> MA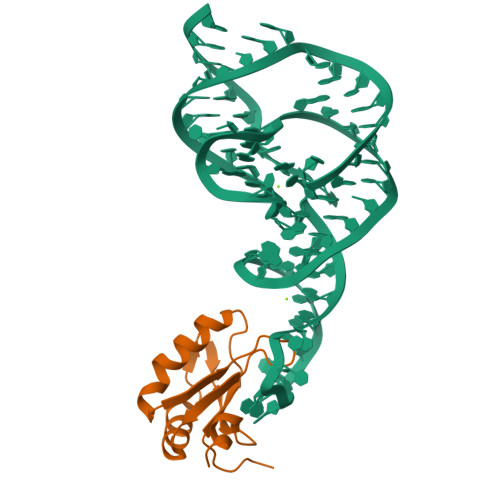VPETRPNHTIYINNLNEKIKKDELKKSLHAIFSRFGQILDILVSRSLKMRGQAFVIFKEVSSATNALRSMQGFPFYDKPMRIQYAKTDSDIIAKMKGT N-[(1S,2R)-1-BENZYL-2-HYDROXY-3-{[3-(TRIFLUOROMETHYL)BENZYL]AMINO}PROPYL]-4-ETHYL-8-(2-OXOPYRROLIDIN-1-YL)QUINOLINE-6-CARBOXAMIDE 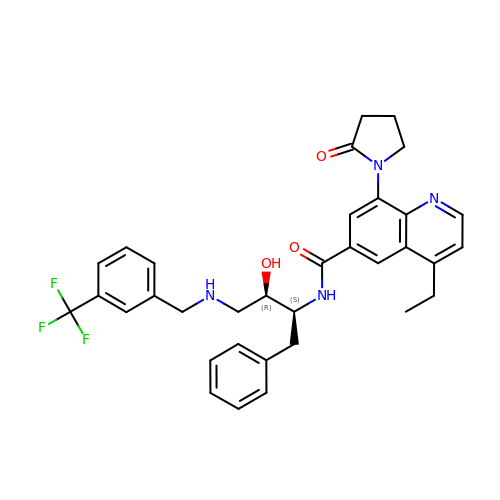| C34 H35 F3 N4 O3 | YDNCUOPJVVQEMT-MFMCTBQISA-N> SAEKLFTPLKVGAVTAPNRVFMAPLTRLRSIEPGDIPTPLMGEYYRQRASAGLIISEATQISAQAKGYAGAPGLHSPEQIAAWKKITAGVHAEDGRIAVQLYHTGRISHSSIQPGGQAPVSASALNANTRTSLRDENGNAIRVDTTTPRALELDEIPGIVNDFRQAVANAREAGFDLVELHSAHGYLLHQFLSPSSNQRTDQYGGSVENRARLVLEVVDAVCNEWSADRIGIRVSPIGTFQNVDNGPNEEADALYLIEELAKRGIAYLHMSETDLAGGKPYSEAFRQKVRERFHGVIIGAGAYT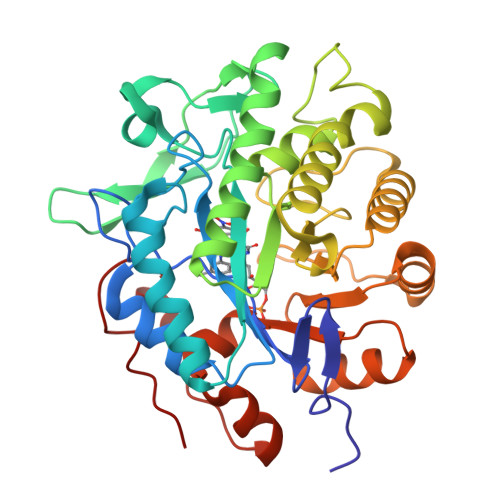AEKAEDLIGKGLIDAVAFGRDYIANPDLVARLQKKAELNPQRPESFYGGGAEGYTDYPSL> MGFKVKLEKRRNAINTCLCIGLDPDEKDIENFMKNEKENNYNNIKKNLKEKYINNVSIKKDILLKAPDNIIREEKSEEFFYFFNHFCFYIIN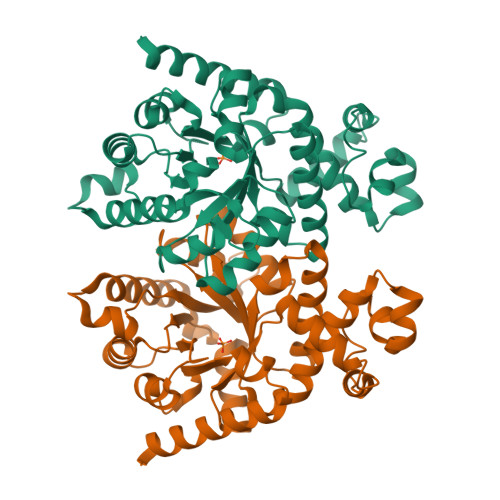ETNKYALTFKMNFAFYIPYGSVGIDVLKNVFDYLYELNIPTILDMKINDIGNTVKNYRKFIFEYLKSDSCTVNIYMGTNMLKDICYDEEKNKYYSAFVLVKTTNPDSAIFQKNLSLDNKQAYVIMAQEALNMSSYLNLEQNNEFIGFVVGANSYDEMNYIRTYFPNCYILSPGIGAQNGDLHKTLTNGYHKSYEKILINIGRAITKNPYPQKAAQMYYDQINAILKQNMES> SKMSDVK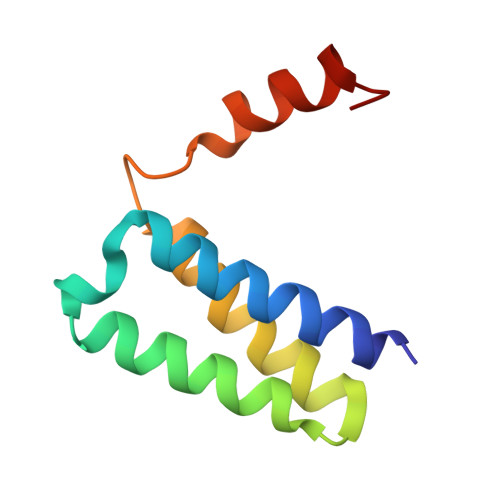CTSVVLLSVLQQLRVESSSKLWAQCVQLHNDILLAKDTTEAFEKMVSLLSVLLSMQGAVDINKLCEEMLDNRATL>[2x]MAVPSLWPWGACLPVIFLSLGFGLDTVEVCPSLDIRSEVAELRQLENCSVVEGHLQILLMFTATGEDFRGLSFPRLTQVTDYLLLFRVYGLESLRDLFPNLAVIRGTRLFLGYALVIFEMPHLRDVALPALGAVLRGAVRVEKNQELCHLSTIDWGLLQPAPGANHIVGNKLGEECADVCPGVLGAAGEPCAKTTFSGHTDYRCWTSSHCQRVCPCPHGMACTARGECCHTECLGGCSQPEDPRACVACRHLYFQGACLWACPPGTYQYESWRCVTAERCASLHSVPGRASTFGIHQGSCLAQCPSGFTRNSSSIFCHKCEGLCPKECKVGTKTIDSIQAAQDLVGCTHVEGSLILNLRQGYNLEPQLQHSLGLVETITGFLKIKHSFALVSLGFFKNLKLIRGDAMVDGNYTLYVL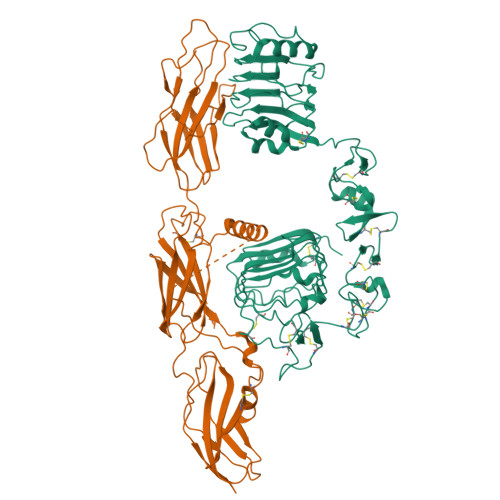DNQNLQQLGSWVAAGLTIPVGKIYFAFNPRLCLEHIYRLEEVTGTRGRQNKAEINPRTNGDRAACQTRTLRFVSNVTEADRILLRWERYEPLEARDLLSFIVYYKESPFQNATEHVGPDACGTQSWNLLDVELPLSRTQEPGVTLASLKPWTQYAVFVRAITLTTEEDSPHQGAQSPIVYLRTLPAAPTVPQDVISTSNSSSHLLVRWKPPTQRNGNLTYYLVLWQRLAEDGDLYLNDYCHRGLRLPTSNNDPRFDGEDGDPEAEMESDCCPCQHPPPGQVLPPLEAQEASFQKKFENFLHNAITIPISPWKVTSINKSPQRDSGRHRRAAGPLRLGGNSSDFEIQEDKVPRERAVLSGLRHFTEYRIDIHACNHAAHTVGCSAATFVFARTMPHREADGIPGKVAWEASSKNSVLLRWLEPPDPNGLILKYEIKYRRLGEEATVLCVSRLRYAKFGGVHLALLPPGNYSARVRATSLAGNGSWTDSVAFYILGPEEEDAGGLHVLLTATPVGLTLLIVLAALGFFYGKKRNRTLYASVNPEYFSASDMYVPDEWEVPREQISIIRELGQGSFGMVYEGLARGLEAGEESTPVALKTVNELASPRECIEFLKEASVMKAFKCHHVVRLLGVVSQGQPTLVIMELMTRGDLKSHLRSLRPEAENNPGLPQPALGEMIQMAGEIADGMAYLAANKFVHRDLAARNCMVSQDFTVKIGDFGMTRDVYETDYYRKGGKGLLPVRWMAPESLKDGIFTTHSDVWSFGVVLWEIVTLAEQPYQGLSNEQVLKFVMDGGVLEELEGCPLQLQELMSRCWQPNPRLRPSFTHILDSIQEELRPSFRLLSFYYSPECRGARGSLPTTDAEPDSSPTPRDCSPQNGGPGH> MAKIYKDEDISLE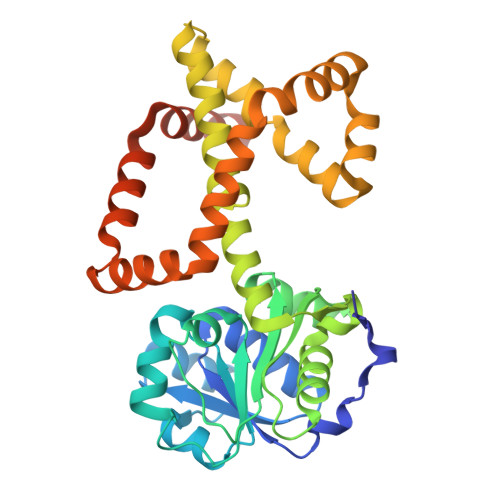PIKNKTIAILGYGSQGRAWALNLRDSGLNVVVGLERQGDSWRRAIDDGFKPMYTKDAVAIADIIVFLVPDMVQKSLWLNSVKDFMKKGADLVFAHGFNIHFKIIEPPKDSDVYMIAPKSPGPIVRRSYEMGGGVPALVAVYQNVSGEALQKALAIAKGIGCARAGVIESTFKEETETDLFGEQVILVGGIMELIKASFETLVEEGYQPEVAYFETVNELKLIVDLIYEKGLTGMLRAVSDTAKYGGITVGKFIIDKSVRDKMKIVLERIRSGEFAREWIKEYERGMPTVFKELSELEGSTIETVGRKLREMMFRGMKQISSHLEHHHHHH> MKLQKQLLEAVEHKQLRPLDVQFALTVAGDEHPAVTLAAALLSHDAGEGHVCLPLSRLENNEASHPLLATCVSEIGELQNWEECLLASQAVSRGDEPTPMILCGDRLYLNRMWCNERTVARFFNEVNHAIEVDEALLAQTLDKLFPVSDEINWQKVAAAVALTRRISVISGGPGTGKTTTVAKLLAALIQMADGERCRIRLAAPTGKAAARLTESLG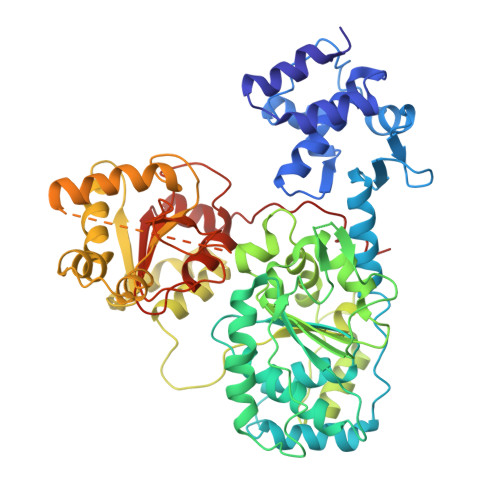KALRQLPLTDEQKKRIPEDASTLHRLLGAQPGSQRLRHHAGNPLHLDVLVVDEASMIDLPMMSRLIDALPDHARVIFLGDRDQLASVEAGAVLGDICAYANAGFTAERARQLSRLTGTHVPAGTGTEAASLRDSLCLLQKSYRFGSDSGIGQLAAAINRGDKTAVKTVFQQDFTDIEKRLLQSGEDYIAMLEEALAGYGRYLDLLQARAEPDLIIQAFNEYQLLCALREGPFGVAGLNERIEQFMQQKRKIHRHPHSRWYEGRPVMIARNDSALGLFNGDIGIALDRGQGTRVWFAMPDGNIKSVQPSRLPEHETTWAMTVHKSQGSEFDHAALILPSQRTPVVTRELVYTAVTRARRRLSLYADERILSAAIATRTERRSGLAALFSSRE(5S,6S,8R)-2-(1,3-benzothiazol-5-yl)-6-hydroxy-4,5,6,7,8,9-hexahydro-5,8-methanopyrazolo[1,5-a][1,3]diazocine-3-carboxamide 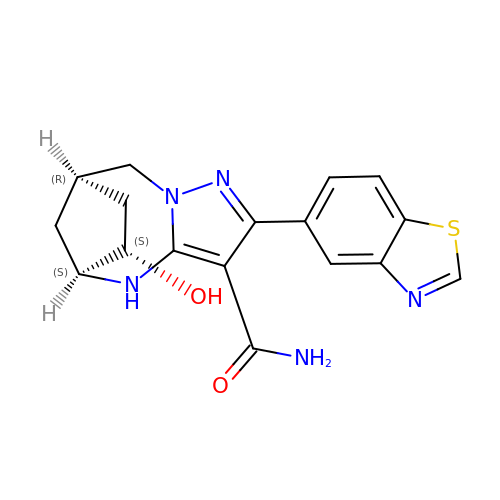| C17 H17 N5 O2 S | IYLHBITVRJLWLH-QRTLGDNMSA-N> MQLLLSEAVSRAAKAAGARPLTSPESLSRDLE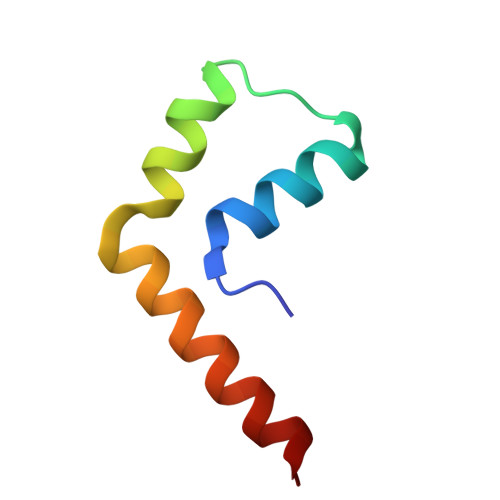APEVQESYRQQLRSDIQKRLQ>MCQTCRVGKRRDAREQIEAKIVELGRRQLLDHGAAGLSLRAIARNLGMVSSAVYRYVSSRDELLTLLLVDAYSDLADTVDRARDDTVADSWSDDVIAIARAVRGWAVTNPARWALLYGSPVPGYHAPPDRTAGVATRVVGAFFDAIAAGIATGDIRLTDDVAPQPMSSDFEKIRQEFGFPGDDRVVTKCFLLWAGVVG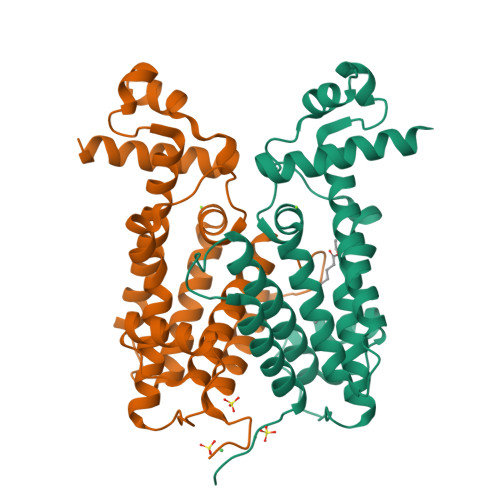AISLEVFGQYGADMLTDPGVVFDAQTRLLVAVLAEHHHHHH[2x]>MGHHHHHHMQATLHQLKVFEATARHGSFTRAAEELYITQPTVSSQIKQLSKTVGLPLFEQIGKRLY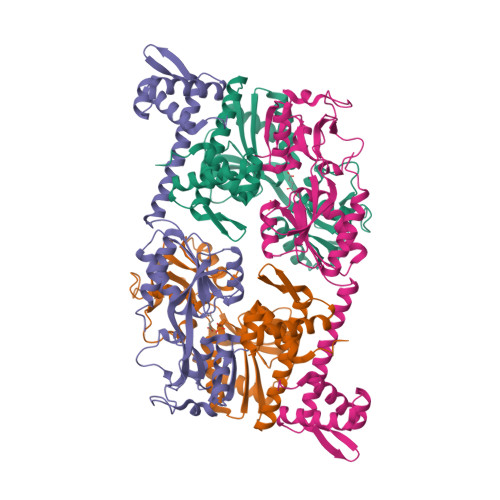LTEAGQELLVTCQDIFQRLDNFAMKVADIKGTKQGRLRLAVITTAKYFIPRLLGEFIQKYPGIEVSLKVTNHEQIRHRMQNNEDDLYIVSEPPEEIDLNYQPFLDNPLVVIARRDHPLAGKSNIPITALNDEAFIMREKGSGTRLAVQNLFHRHYVDVRVRLELGSNEAIKQAIAGGMGISVLSQHTLVSEGARSELTILDIDEFPIKRRWYVANLAGKQLSVITQTFLDYLMAVTKNMPAPFAEQLTTQQTPVKLVL[4x]> MRGSHHHHHHGSMSQISRGLENVFIKTTSLTYID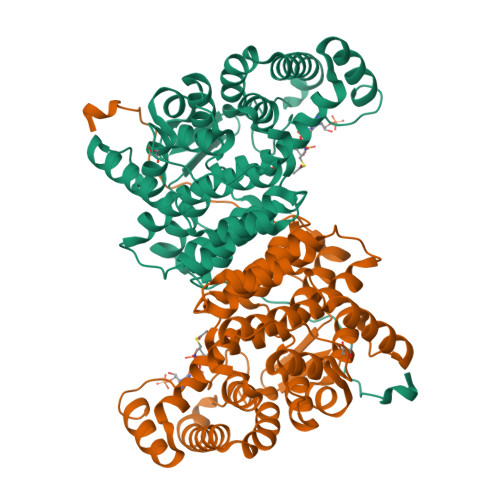GENGILRYGGYDIEDLVEHTSFEEVVHLMLYGDLPTKLQLQRLKSALDEAYEVPQQVIDMIYSLPRDSDAVGMMETAFSALSSIYGMPWNKATNRDNAVKLVARASTVVANVLRAKEGKKPAIPEPSESFAKSFLKASFSRTPTEEEVKAMDAALILYADHEVPASTTAALVTSSTLSDIYSCVVAALAALKGPLHGGAAEEAFKQFVEIGEPDMTESWFKRKIIEGKSRLMGFGHRVYKTYDPRAKIFKKYAKVISERNSDARKYFEIAQKLEELGVETFGAKHIYPNTDFYSGVVFYALGFPVYMFTSLFALSRTLGWTAHVIEYVEDQHRLIRPRALYVGPLKRDVVPIELRG> SGTVTFDITNIDWETAEWIMKHVYLIAKKEGTDVTFSFKEGELQITVKNLHEEAKREIEKWIRAAQLAQDPDAESKAEARKILNELITEKAEELREKTKDEEVRELAREAARLALESDDIEVQRVVLKALLAALKSKDEEVIRLLLLAAVLAAAAARSGSPEEKLEIAKKALELAMKSKDEEVIRLALLAAVLAARSDDEEVLKKVKEALEKMERIMDLEDVAREKSGSAEASQAVKEIADIAEEALREGLCEVARVALKRLFKLAKDYPGSDVASLAKKALEKIAETALRNGCKETAE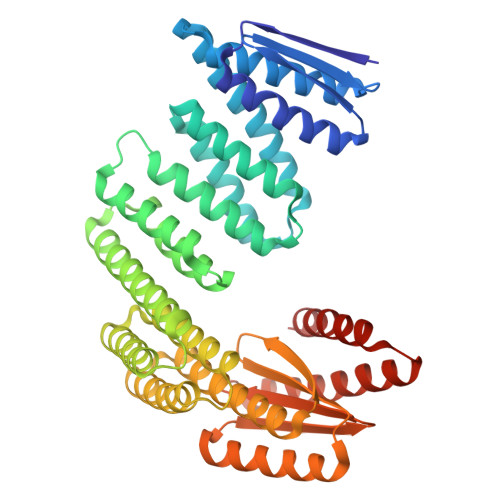LAKLLLFLLLIIEVVLKMGVRMLTHRGGNAVIVVIEGLHPSQIVQLMQDVIKAAKKLGVTVTITVSGDIVVIMVVVGASDEEQEEARRLVQEIARALQEAKRKGANEEQLEQLLRELLERAEREGGSG>MTDVKKSIRANRGTELECLGWEQEAVLRMLRNNLDPEVAEKPEDLIVYGGIGKAARDWDAFHAIEHSLKTLKNDETLLVQSGKPVGMFRTHPQAPRV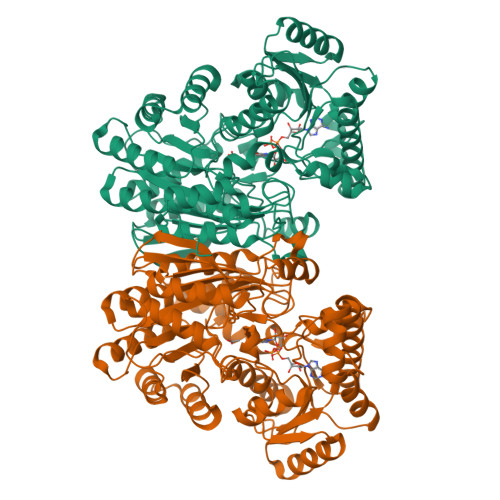LLANSVLVPKWADWEHFHELEKKGLMMYGQMTAGSWIYIGSQGILQGTYETFAELARQHFGGSLKGTLTLTAGLGGMGGAQPLSVTMNEGVVIAVEVDEKRIDKRIETKYCDRKTASIEEALAWAEEAKLAGKPLSIALLGNAAEVHHTLLNRGVKIDIVTDQTSAHDPLIGYVPEGYSLDEADRLRQDTPELYVRLAKQSMKKHVEAMLAFQQKGSIVFDYGNNIRQVAKDEGLENAFDFPGFVPAYIRPLFCEGKGPFRWAALSGDPADIYRTDALLKELFPTNKALHRWIDMAQEKVTFQGLPSRICWLGYGERKKMGLAINELVRTGELKAPVVIGRDHLDCGSVASPNRETEAMKDGSDAVGDWAVLNALVNTAAGASWVSFHHGGGVGMGYSLHAGMVAVADGSELADERLARVLTSDPGMGIIRHADAGYERAVEVAKEQDIIVPMQK[4x]> MGHHHHHHSHMNEDIHFEPIVSLPEVEVKSGEEDEEILFKERAKLYRWDRDVSQWKERGVGDI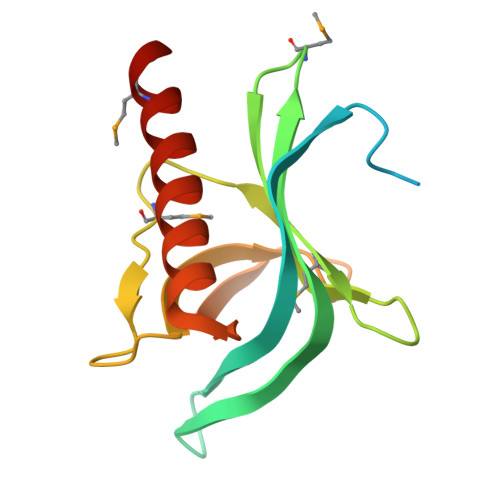KILWHTMKNYYRILMRRDQVFKVCANHVITKTMELKPLNVSNNALVWTASDYADGEAKVEQLAVRFKTKEVADCFKKTFEECQQNLMKLQKG>[4x]MGSSHHHHHHENLYFQSDPRFPLTARDKFSLVKSWKTFSRNLESAGKEMLLKLFIEHPDMKDLFPKFKAKTPDQLRNDESFEEAALAHITPYDQAVQDSDNVDILLTNLKRVGRQHKTV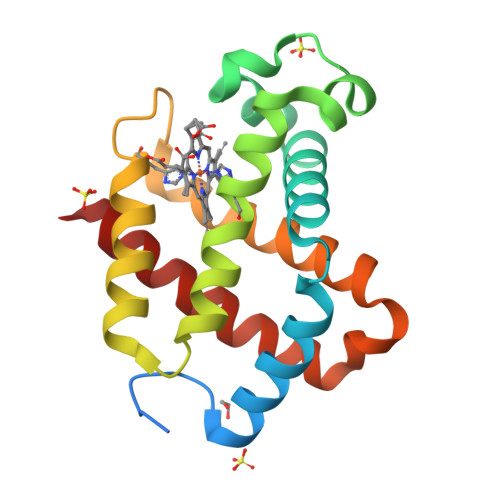PGFQESYFERMEKCLVFALQTTLADAYTENMERIYKIWISWTTEKIREGFRE> GGAGGGAAAAGUUAUCAGGCAUGCACCUGGUAGCUAGUCUUUAAACCAAUAGAUUGCAUCGGUUUAAAAGGCAAGACCGUCAAAUUGCGGGAAAGGGGUCAACAGCCGUUCAGUACCAAGUCUCAGGGGAAACUUUGAGAUGGCCUUGCAAAGGGUAUGGUAAUAAGCUGACGGACAUGGUCCUAACCACGCAGCCAAGUCCUAAGUCAACAGAUCUUCUGUUGAUAUGGAUGCAGUUCACAGACUAAAUGUCGGUCGGGGAAGAUGUAUUC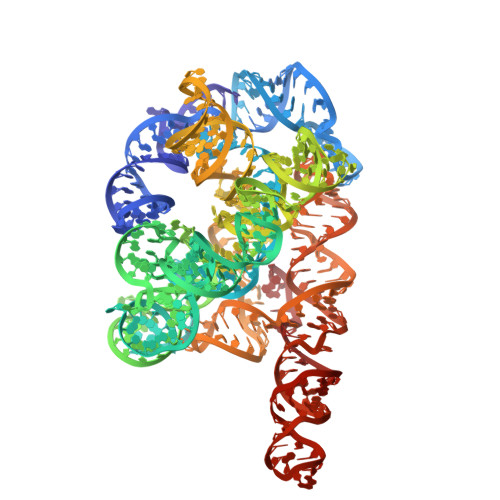UUCUCAUAAGAUAUAGUCGGACCUCUCCUUAAUGGGAGCUAGCGGAUGAAGUGAUGCAACACUGGAGCCGCUGGGAACUAAUUUGUAUGCGAAAGUAUAUUGAUUAGUUUUGGAGU>[4x]VDFKLSPSQLEARRHAQAFANTVLTKASAEYSTQKDQLSRFQATRPFYREAVRHGLIKAQVPIPLGGTMESLVHESIILEELFAVEPATSITIVATALGLMPVILCDSPSLQEKFLKPFISGEGEPLASLMHSEPNGTANWLQKGGPGLQTTARKVGNEWVISGEKLWPSNSGGWDYKGADLACVVC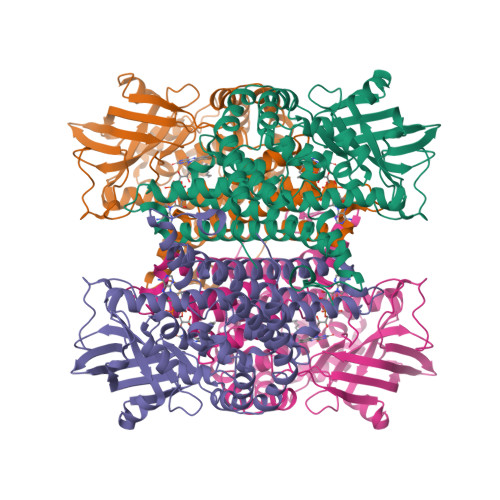RVSDDPSKPQDPNVDPATQIAVLLVTRETIANNKKDAYQILGEPELAGHITTSGPHTRFTEFHVPHENLLCTPGLKAQGLVETAFAMSAALVGAMAIGTARAAFEEALVFAKSDTRGGSKHIIEHQSVADKLIDCKIRLETSRLLVWKAVTTLEDEALEWKVKLEMAMQTKIYTTDVAVECVIDAMKAVGMKSYAKDMSFPRLLNEVMCYPLFNGGNIGLRRRQMQRVMALEDYEPWAATYGSSKVDKSRL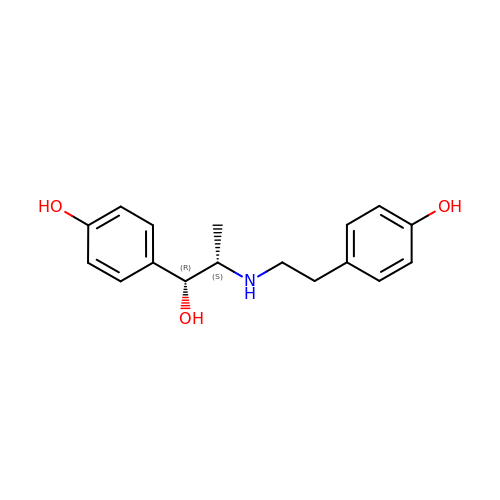4-[(1R,2S)-1-hydroxy-2-{[2-(4-hydroxyphenyl)ethyl]amino}propyl]phenol | C17 H21 N O3 | IOVGROKTTNBUGK-SJCJKPOMSA-N>[2x]FADDHAMSPDMKLLAGASNWVNQSGSVAQFVFTPSPTQPQTYEVSGNYINNAQGTGCKGTPYPLSGAYYSGNQIISFSVVWSNASANCQSATGWTGYFDFSGSQAVLKTDWNLA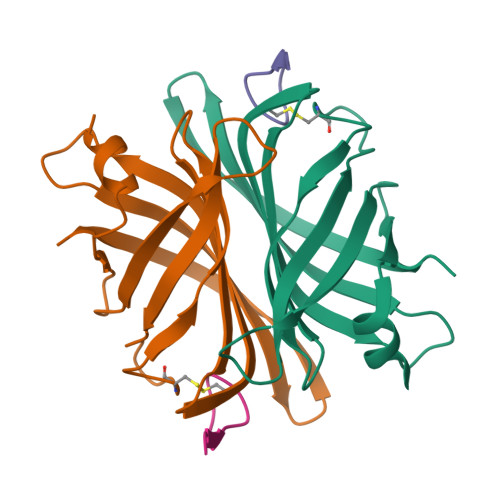FYSGSTPAIQQGQDDFMQSV;>[2x]SVATVSESLLTE>[2x]HHHHHHMASSAQDGNNPLFSPYKMGKFNLSHRVVLAPMTRCRALNNIPQAALGEYYEQRATAGGFLITEGTMISPTSAGFPHVPGIFTKEQVREWKKIVDVVH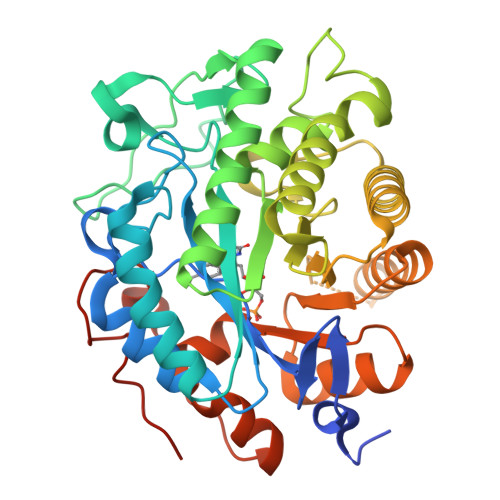AKGAVIFCQLWHVGRASHEVYQPAGAAPISSTEKPISNRWRILMPDGTHGIYPKPRAIGTYEISQVVEDYRRSALNAIEAGFDGIEIHGAHGYLIDQFLKDGINDRTDEYGGSLANRCKFITQVVQAVVSAIGADRVGVRVSPAIDHLDAMDSNPLSLGLAVVERLNKIQLHSGSKLAYLHVTQPRYVAYGQTEAGRLGSEEEEARLMRTLRNAYQGTFICSGGYTRELGIEAVAQGDADLVSYGRLFISNPDLVMRIKLNAPLNKFNRKTFYTQDPVVGYTDYPFLQGNGSNGPLSRL> MAAKGDMLYAWAKDAEIQKKGECGGAVTALLKHALETKMVDAVVAIKKGKDLYDAVPTVITNPEDIIQTAGSLHCGTLLIPKLIKKYLNGAKDMKLAVTCKGCDAMAFYELAKRNQINLDNIIMIGVNCGGSVSPVTARKMISNKFGVDPDTVHKEEIDKGQFIIEYEGGHKGIKIDELEEEGYGRRSNCRRCKMKIPRQADIAAGNWGVIGDKAGKATFLEICSEKGANLVNSAQSKGALEISPADPKGIDIRAKVEKAMFNLGDEWRHRDF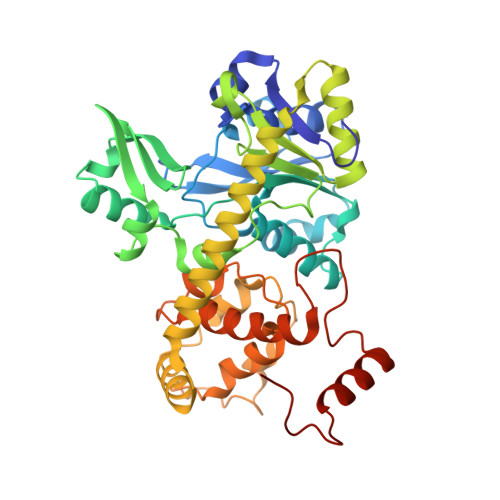EGMGKGKDRLKLMMSESSKCIKCYACVEACPICYCIECSTKKPWYIAPGVLPTSFMFHLIRFAHVSDSCINCGQCEELCPMEIPNALFMHSQQVEIEKMFGHIPGQDMTPPIHAFVEEKAERARLDATGTDSIYTNIFTDE>NRINVFKTNGFSKSLGEHRMTSKVLVFKEMATPPKSVQDELQLNADDTVYYLERLRFVDDDVLCIEYSYYHKEIVKYLNDDIAKGSIFDYLESNMKLRIGFSDIFFNVDKLTSSEASLLQLSTGEPCLRYHQTFYTMTGKPFD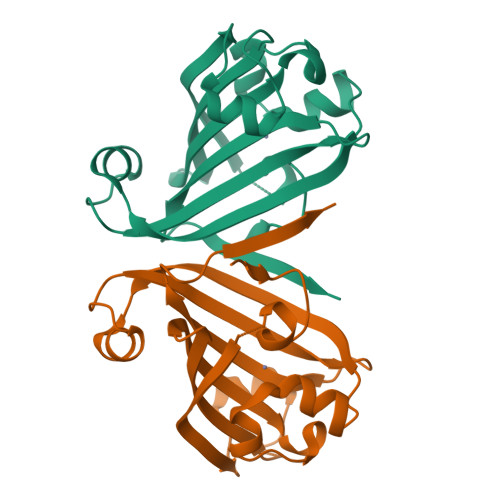SSDIVFHYRHAQFYIPSKK[2x]1-{[2-(difluoromethoxy)phenyl]methyl}-2-methyl-6-[6-(piperazin-1-yl)pyridin-3-yl]-1H-benzimidazole 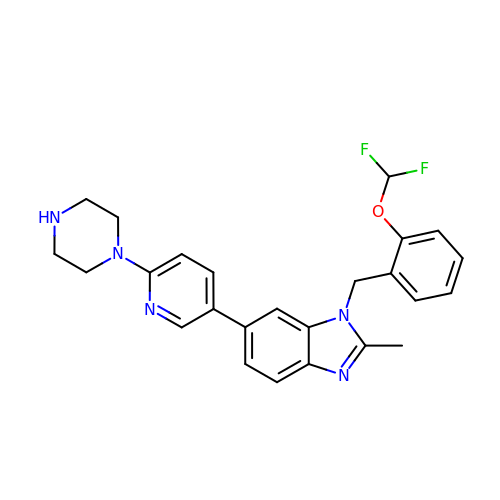| C25 H25 F2 N5 O | LRHACCJNWLLTDS-UHFFFAOYSA-N> VDLVFLFDGSMSLQPDEFQKILDFMKDVMKKCSNTSYQFAAVQFSTSYKTEFDFSDYVKRKDPDALLKHVKHMLLLTNTFGAINYVATEVFREELGARPDATKVLIIITDGEATDSGNIDAAKDIIR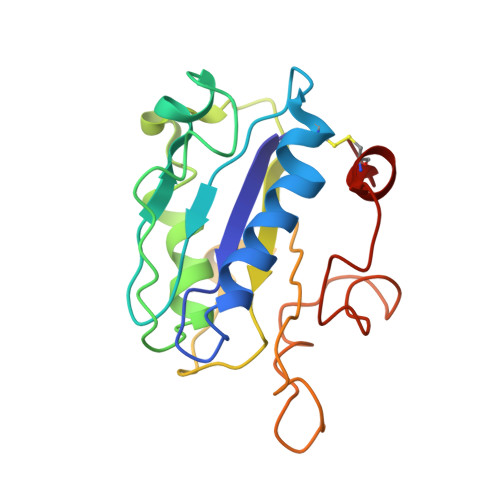YIIGIGKHFQTKESQETLHKFASKPASEFVKILDTFEKLKDLCTELQKKI> MTAGLLEAPTADWVHLADLYQNPFPIFERLRSESPVAWVPEAGRYLITSYSGVLAADVDQTTFSANEKKSLMLRAMGHSMLRKDDPDHQVERRAWQPSLKPGTVKKVWKQKFAENADRYLDAYIDAGSGSDFMQGFAAPFVAENLRALIGFENASEADLQRWSQTLIDGAGNYPDDPDVWAKAKQSSDEIDAALEEMIQWHSGRPGD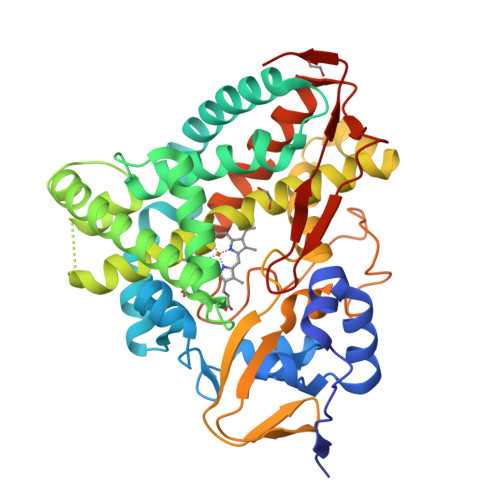SLLSYLLRSADYQMPLESIRSNIKMTIGGGLNEPRDVLGVSTLALLSSSKQLELVLRDPKLWGAVFEESIRWVAPIGMVPRQTVVDTELDGYFIPRGAKLGLCILSANRDRSVWSDPDRFDIERGSEAHLAFGKGVHVCLGAWAARSQVADVGLPALFSRLKGLRLDPNQEATHGGWVFRGPLSLPLVWDKAVRSELA>MTSAEMTSPNNNSEHQAIAKMRTMIEGFDDISHGGLPIGRSTLVSGTTGTGKTLFSIQFLYNGIIEFDEPGVFVTFEETPQDIIKNARSFGWDLAKLVDEGKLFILDASPDPEGQEVVGGFDLSALIERINYAIQKYRARRVSIDSVTSVFQQYDASSVVRRELFRLVARLKQIGATTVMTTERIEEYGPIARY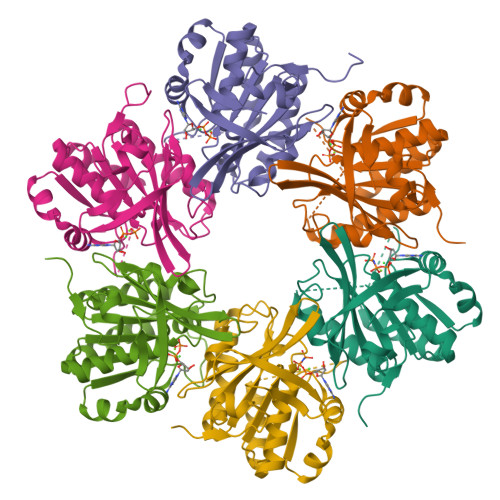GVEEFVSDNVVILRNVLEGERRRRTLEILKLRGTSHMKGEYPFTITDHGINIFPLGAMR[6x]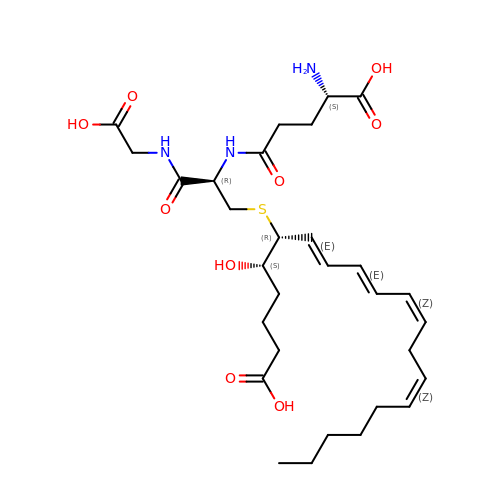(5~{S},6~{R},7~{E},9~{E},11~{Z},14~{Z})-6-[(2~{R})-2-[[(4~{S})-4-azanyl-5-oxidanyl-5-oxidanylidene-pentanoyl]amino]-3-(2-hydroxy-2-oxoethylamino)-3-oxidanylidene-propyl]sulfanyl-5-oxidanyl-icosa-7,9,11,14-tetraenoic acid | C30 H47 N3 O9 S | GWNVDXQDILPJIG-NXOLIXFESA-N One well conserved pathway that it shares with other bacterial pathogens is for fatty-acid biosynthesis as a primary source of cell-membrane lipids. In R. prowazekii fatty-acid biosynthesis occurs via the type II fatty-acid synthase pathway, which is thought to be descendant from an algal plastid and consists of four to eight individual enzymes that start with acetyl coenzyme A and malonyl-(acyl-carrier-protein) to create elongated fatty acids for the lipid bilayer. Thus, unlike other members of the short-chain dehydrogenase/reductase superfamily, FabG undergoes a substantial conformational change upon cofactor binding that organizes the active-site triad (Ser143, Tyr156 and Arg160) and alters the affinity of the other substrate-binding sites in the tetrameric enzyme. While a number of antimicrobial options have been identified for targeting most of the enzymes in the FAS II pathway, FabG is still relatively unaddressed, in part owing to the conformational change that it undergoes.

The SSGCID has solved a 2.25 Å resolution structure of R. prowazekii FabG, a 3-ketoacyl-(acyl-carrier-protein) reductase, which corresponds well to the solved structures for other notable bacterial pathogens while differing from mammalian analogs. For Rickettsia in particular this is a significant target for drug development as the organism has a minimal proteome with very few essential biosynthetic pathways maintained. The structure of R. prowazekii FabG is very similar to those reported for E. coli FabG and other bacterial FabGs; the protomer assumes a Rossmann-fold structure with a seven β-­stranded twisted parallel β-sheet flanked by four α-helices on either side and two βαβαβ motifs at the core. R. prowazekii FabG crystallizes with two protomers per asymmetric unit. A tetramer is generated by crystallographic symmetry. For FabGs tetramers are typically observed. It is therefore assumed that R. prowazekii FabG is in a tetrameric state. Based on these high overall correspondences in sequence and secondary and tertiary structure, conclusions drawn from the other bacterial structures may also be applicable to the Rickettsia protein. Owing to a significant conformational change during substrate binding, it has been difficult to identify suitable inhibitors for this essential and highly conserved enzyme.

>MAHHHHHHMIDLTGKTSLITGASSGIGSAIARLLHKLGSKVIISGSNEEKLKSLGNALKDNYTIEVCNLANKEECSNLISKTSNLDILVCNAGITSDTLAIRMKDQDFDKVIDINLKANFILNREAIKKMIQKRYGRIINISSIVGIAGNPGQANYCASKAGLIGMTKSLSYEVATRGITVNAVAPGFIKSDMTDKLNEKQREAIVQKIPLGTYGIPEDVAYAVAFLASNNASYITGQTLHVNGGMLMV[2x]(3~{a}~{S})-2-[(3~{S})-1-azabicyclo[2.2.2]octan-3-yl]-3~{a},4,5,6-tetrahydro-3~{H}-benzo[de]isoquinolin-1-one 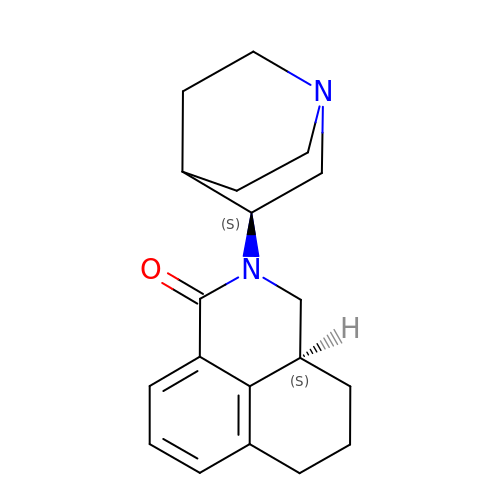| C19 H24 N2 O | CPZBLNMUGSZIPR-NVXWUHKLSA-N>SATLTAKNLAKAYKGRRVVEDVSLTVNSGEIVGLLGPNGAGKTTTFYMVVGIVPRDAGNIIIDDDDISLLPLHARARRGIGYLPQEASIFRRLSVYDNLMAVLQIRDDLSAEQREDRANELMEEFHIEHLRDSMGQSLSGGERRRVEIARALAANPKFILLDQPFAGVDPISVIDIKRIIEHLRDSGLGVLITDHNVRETLAVCERAYIVSQ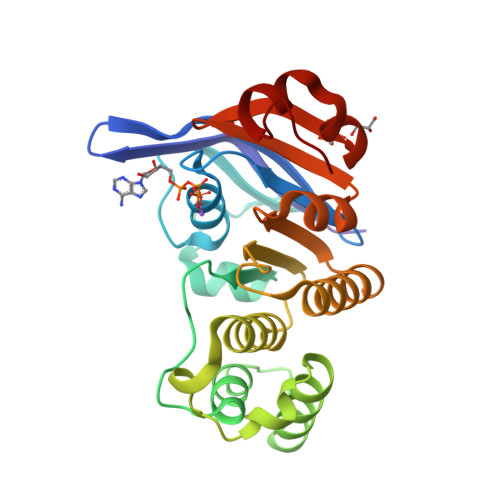GHLIAHGTPTEILQDEHVKRVYLGEDFRL[2x]> AGWNVNSKQN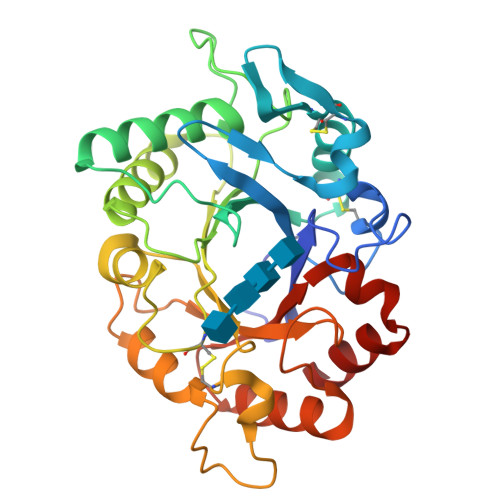IAVYWGQNSANSQSTQQRLSFYCNDANINVIDIAFLNGITPPMTNFANAGDRCTPFSDNPWLLQCPEIEADIKTCQANGKTILLSLGGDSYTQGGWSSTGAAQSAADQVWAMFGPVQSGSSVHRPFGSAVVDGFDFAFAATTNNLAAFGAQLKSRTNAAGGKKYYFSAAPQCFFPDAAVGALINAVPMDWIQIQFYNNPCGVSGFTPGTSTQNNYNYQTWENWAKTSPNPNVKLLVGIPAGPGAGRGYVSGSQLTSVFQYSKGFSTFAGAMMWDMSQLYQNTGFETQVVNALR At the cell division site, FtsZ protofilaments form a highly dynamic, membrane-bound structure, the Z-ring, which serves as a scaffold for the recruitment of the extra-cytoplasmic cell wall biosynthetic machinery. Here we investigate the physiological function of Corynebacterium glutamicum SepF, the only cell division-associated protein from Actinobacteria known to interact with the conserved C-terminal tail of FtsZ. Our structural data revealed the FtsZ-binding pocket, defining the SepF homodimer as the functional unit, and suggesting a reversible β-sheet-mediated oligomerization interface possibly regulated via an alpha helical switch. We found that FtsZ filaments and lipid membranes have opposing effects on SepF polymerization, pointing to a complex dynamic role of the protein at the division site, involving FtsZ bundling, Z-ring tethering and membrane reshaping activities that are needed for proper Z-ring assembly and function.

To elucidate the structural basis of FtsZ recognition, we crystallized the SepF C-terminal core domain (SepFΔML) in complex with a 10-residues peptide comprising the conserved C-terminal domain (CTD) of FtsZ (FtsZCTD) and determined the crystal structure at 1.6 Å resolution. The SepF structure revealed a symmetric homodimer, with monomers that contain a central four-stranded β-sheet stacked against two α-helices (α1, α2) involved in dimerization and capped by a C-terminal α-helix (α3) on the opposite side of the sheet. The homodimer contains two identical FtsZCTD-binding pockets, each made up of residues coming from both protomers, defining a dimeric functional unit for the SepF–FtsZ interaction. This 2:2 binding stoichiometry can explain mechanistically why B. subtilis SepF has a bundling effect on FtsZ protofilaments. The bound FtsZCTD is clearly visible in the electron density map, and adopts a hook-like extended conformation that fits into a mostly hydrophobic binding pocket formed by conserved SepF residues, where it is further stabilized by additional intermolecular hydrogen-bonding interactions. The SepF-bound structure of the FtsZCTD peptide revealed yet another non-helical conformation, reflecting the large conformational space that this small, highly conserved sequence can adopt in different biological contexts. It is interesting to note that SlmA and SepF, despite their different structures and binding pockets, interact with the same highly conserved hydrophobic motif of the FtsZCTD. The interface was further validated by mutating two FtsZCTD-contact residues in SepF: F131A and K125E. Compared with the wild-type protein, the single mutant SepFΔML,F131A was greatly compromised for FtsZ binding (apparent Kd = 340 + /− 47 μM), whereas the double mutant SepFΔML,K125E/F131A exhibited no detectable binding in the range of protein-peptide concentrations tested.

>[2x]MSYQSTIVPVELHSFEDAQVIGGAFRDGDAVVFDMSLLSREEARRIVDFAAGLCFALRGKMQKIDSVTFAVVPELSNISTSELERAARIR;>DDLDVPSFLQ[2x]>[4x]PQFSLWKR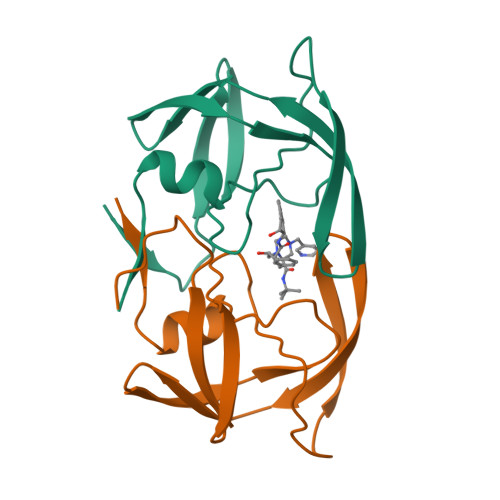PVVTAYIEGQPVEVLLDTGADDSIVAGIELGNNYSPKIVGGIGGFINTKEYKNVEIEVLNKKVRATIMTGDTPINIFGRNILTALGMSLNL> GSHRTSGRVAVEEVDEEGKFV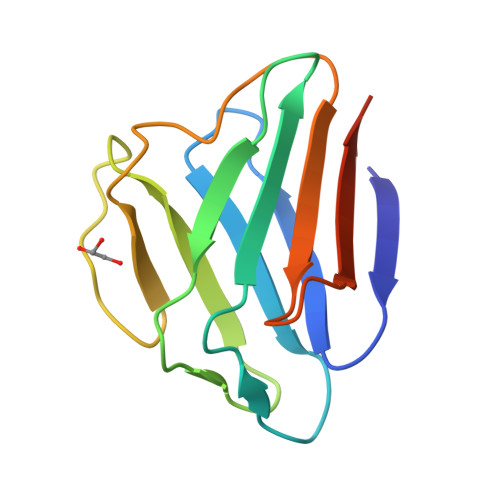RLRNKSNEDQSMGNWQIKRQNGDDPLLTYRFPPKFTLKAGQVVTIWAAGAGATHSPPTDLVWKAQNTWGCGNSLRTALINSTGEEVAMRKLVRSVTVVED> AQSVPYGVSQIKAPALHSQGYTGSNVKVAVIDSGIDSSHPDLKVAGGASMVPSETNPFQDNNSHGTHVAGTVAALNNSIGVLGVAPSASLYAVKVLGADGSGQYSWIINGIEWAIANNMDVINMSLGGPSGSAALKAAVDKAVASGVVVVAAAGNEGTSGSSSTVGYPGKYPSVIAVGAVDSSNQRASFSSVGPELDVMAPGVSIQSTLPGNKYGAYNGTSMASPHVAGAAALILSKHPNWTNTQVRSSLENTTTKLGDSFYYGKGLINVQAAAQHHHHHH;> MKTEWPELVGKSV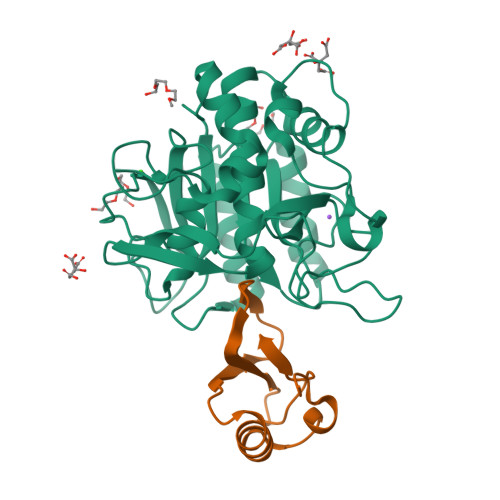EEAKKVILQDKPAAQIIVLPVGTIVTAEYRIDRVRLFVDRLDNIAQVPRVG> PSSSMADFRKFFAKAKHIVIISGAGVSAESGVPTFRGAGGYWRKWQAQDLAT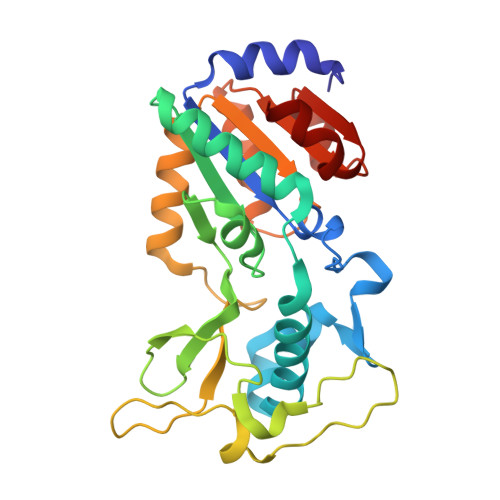PLAFAHNPSRVWEFYHYRREVMGSKEPNAGHRAIAECETRLGKQGRRVVVITQNIDELHRKAGTKNLLEIHGSLFKTRCTSCGVVAENYKSPICPALSGKGAPEPGTQDASIPVEKLPRCEEAGCGGLLRPHVVWFGENLDPAILEEVDRELAHCDLCLVVGTSSVVYPAAMFAPQVAARGVPVAEFNTETTPATNRFRFHFQGPCGTTLPEALA>[6x]SNAMNNTQKKLKVLFIGESWHIHMIHSKGYDSFTSSKYEEGATWLLECLRKGGVDIDYMPAHTVQIAFPESIDELNRYDVIVISDIGSNTFLLQNETFYQLKIKPNALESIKEYVKNGGGLLMIGGYLSFMGIEAKANYKNTVLAEVLPVIMLDGDDRVEKPEGIC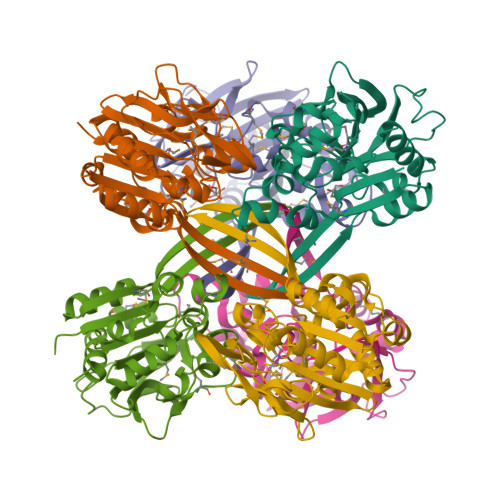AEAVSPEHPVVNGFSDYPVFLGYNQAVARDDADVVLTINNDPLLVFGEYQQGKTACFMSDCSPHWGTQQFMSWPFYTDLWVNTLQFIARK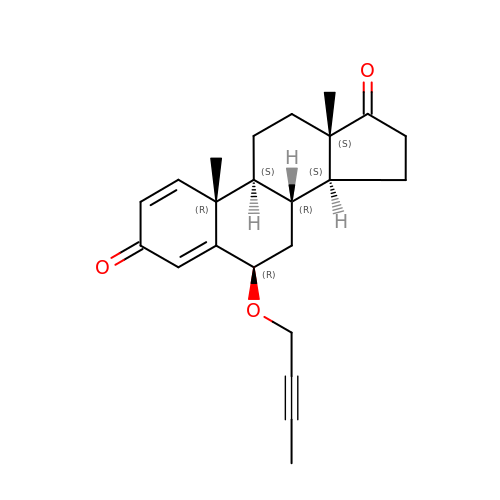(6alpha,8alpha)-6-(but-2-yn-1-yloxy)androsta-1,4-diene-3,17-dione | C23 H28 O3 | GNDYBZKXORBCFO-KVAKACLVSA-N The closely related REV-ERBα and REV-ERBβ proteins generally act as transcriptional repressors, either on their own, by recruiting co-repressor proteins, or by competing with the Retinoid-related Orphan Receptors (RORs) α, β, or γ for the same DNA binding sites. Physiologically, the REV-ERB proteins play a number of diverse and important roles ranging from the control of circadian biology to the homeostasis of lipids. The REV-ERBs also bind heme but, unlike E75, the heme can readily dissociate from the REV-ERBs, and this reversible binding regulates REV-ERB transcription activity. Using transcription assays from native and model promoters in cells, we report that the REV-ERBs are also gas-binding components of the molecular clock and that gas and redox state modulate the structure and function of the REV-ERB LBDs.

To shed light on the structural basis of heme, gas, and redox regulation, we crystallized the REV-ERBβ LBD in the heme-bound state. The formation of well-ordered crystals required the addition of trypsin to the crystallization solution. Two identical structures were obtained using constructs comprising either the complete LBD (residues 212–579) or the LBD with an internal deletion (residues 241–579 Δ 275–357). Both 1.9 Å resolution structures include α-helices 3–11, (residues 381–576; REV-ERBβ381–576), which is slightly larger than the fragment used to derive the unliganded LBD structure. The two REV-ERBβ381–576 Fe(III) heme structures verify that the heme-binding pocket is in fact present at the same position as ligand-binding pockets observed in other NR family members. As predicted by the mutagenesis and spectroscopic analyses for the oxidized state of REV-ERB, a single heme molecule is hexa-coordinated within the pocket by Cys384 and His568 side chains. The structural changes that facilitate heme binding are confined primarily to helices 3, 7, and 11. In the presence of heme, helix 3 straightens, swinging the end of its N-terminal half (Cα atom Gly398) 16.4 Å away from its position in the unliganded structure. To facilitate heme binding, it also undergoes a major conformational change, swinging its C terminus (Cα atom Leu576) 15 Å away from the ligand-binding pocket, forming a gently curving, uninterrupted α-helix that covers the ligand pocket. First, the imidazole side chain of His568 makes a ∼120° rotation around the axis of the helix to allow bonding with the Fe(III) heme center.

> HLVCPMSKSPYVDPHKSGHEIWEEFSMSFTPAVKEVVEFAKRIPGFRDLSQHDQVNLLKAGTFEVLMVRFASLFDAKERTVTFLSGKKYSVDDLHSMGAGDLLNSMFEFSEKLNALQLSDEEMSLFTAVVLVSADRSGIENVNSVEALQETLIRALRTLIMKNHPNEASIFTKLLLKLPDLRSLNNMHSEELLAFKVHP6-(cyclohexylsulfanyl)-1-(ethoxymethyl)-5-(1-methylethyl)pyrimidine-2,4(1H,3H)-dione | C16 H26 N2 O3 S | 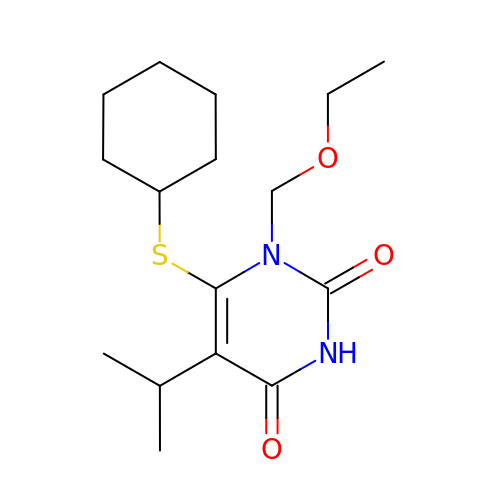JKXLRLDPSLZEDD-UHFFFAOYSA-N>[2x]HHHHHHSSGENLYFQSMQFEKVTYIAVPQKYGQKKVGVEEGPKFLEKLGFMNVLEQVAKSVNKKTITEPKTPQELGVTNARNLNEVESVNIELRDTIAKEYDVNNLLIN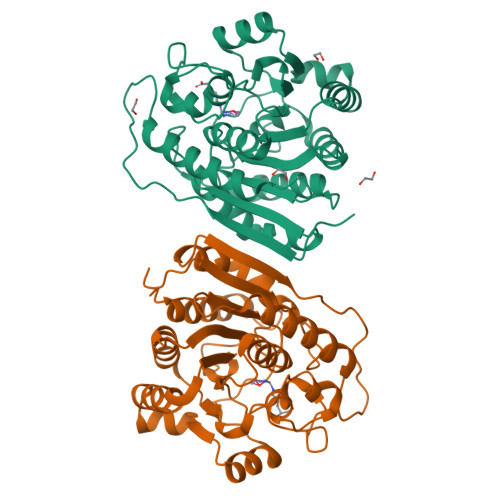IGGDHSIGLGTIAGVVKAMKPNARVGVVWFDAHPDMNTPENSPSGNIHGMPLACAVGLGPQRLTSIMPHYITPKDIMYVGIRSIDVGEQFEIQDKHIDHFTAEDVKRVGMKEVIEAINKKFVDYDVIHLSFDIDGIDPEFILGTGTPVPKGISLEDSLYFMSEMGKMKKLHSVDIVEYNPKIEEEITGKNVLKCISSLFGIKC> MLAKYGDLTVVKDDLTLLEKTESYIAKWRLNRWEFRVPPLLYPAVREKVMLQQEILKALCLNRAEEHK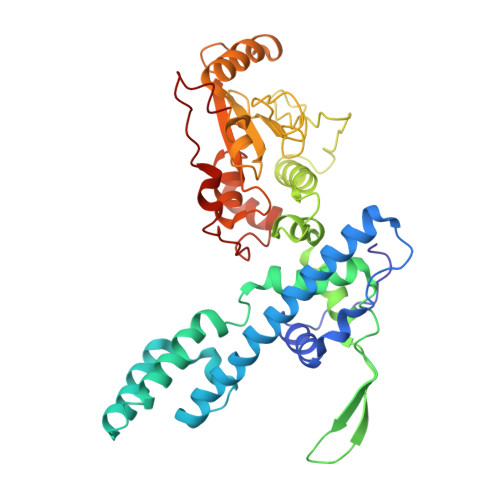HVLGDIQIVASITGISPESVREKNRAWLQEEASKLRWKGEVNKAKELRDAFLRLEVYGSRDHRLLERLCCIYGMGMQGTFDEAFSNIIVQDPSTGKLAVDEANPFAELQAYILSRYPQIDLIHDFLGLNVVSGYRPSLGRFLIHCLSKKNNISNPVSNGRVLLHVSTSKETLFDYGDSKNQVAHDDSIYGLPDFMYVRGNDIFLIIIAADNHWLRKRQVPHTKQLEGIARRCSFVLGIPFDKVRIRNLLLPPNYVDSSSLRRLTETVFDMSPASVKEAVPWISLYEKGLDAQDVDYCELEKTVNEEEWLTL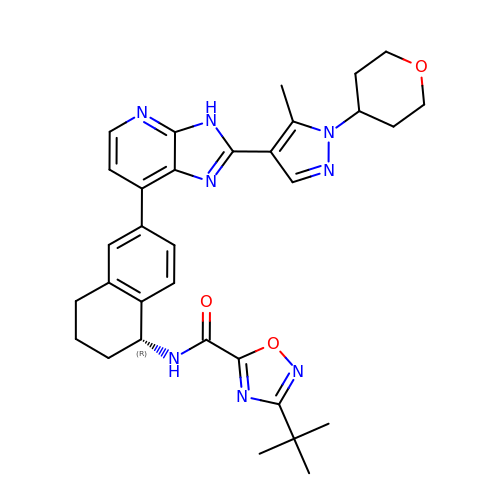3-tert-butyl-N-[(1R)-6-{2-[5-methyl-1-(oxan-4-yl)-1H-pyrazol-4-yl]-3H-imidazo[4,5-b]pyridin-7-yl}-1,2,3,4-tetrahydronaphthalen-1-yl]-1,2,4-oxadiazole-5-carboxamide | C32 H36 N8 O3 | IWJJKWNPIYKQNB-RUZDIDTESA-N>TLKIVWS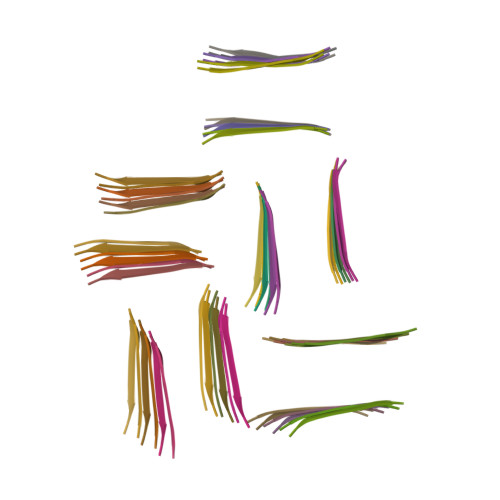[60x]> GKSASGEKEGNENAEEEAAAIEEARREAEERRKEKHRKMEEEREEMRQTIRDKYGLKKKVKEEPEAEADLDEGR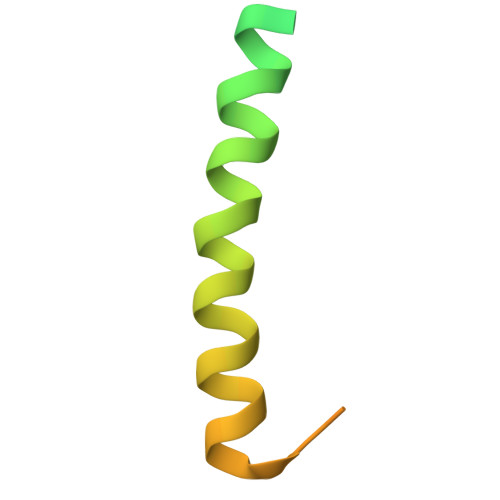VGRKK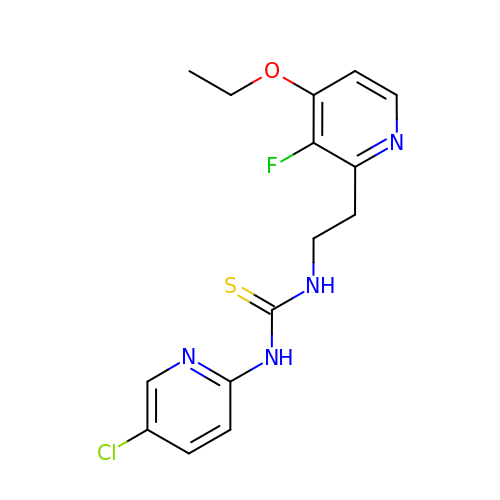N-[[3-FLUORO-4-ETHOXY-PYRID-2-YL]ETHYL]-N'-[5-CHLORO-PYRIDYL]-THIOUREA | C15 H16 Cl F N4 O S | VEBKSFPYWMOUBR-UHFFFAOYSA-N> EASLLSFEKLDRASAD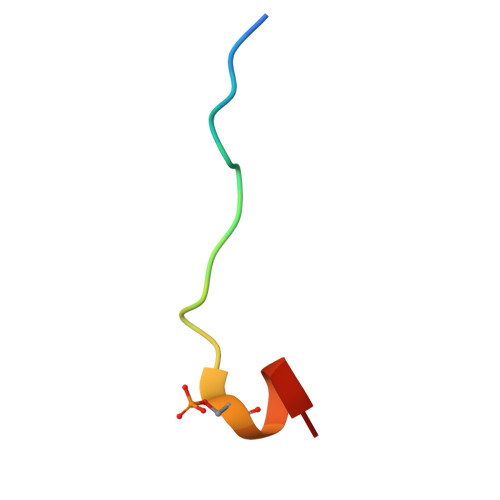LWPE>[2x]EDPEV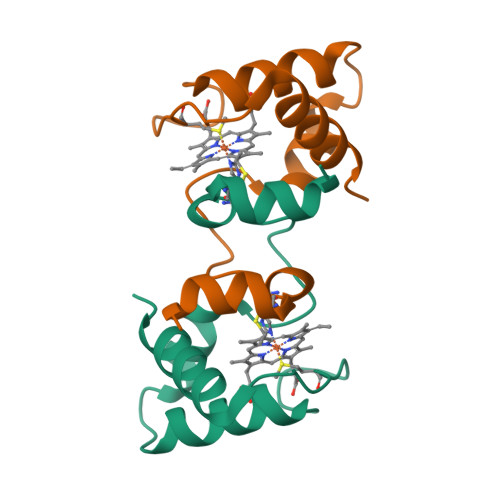LFKNKGCVACHAIDTKMVGPAYKDVAAKFAGQAGAEAELAQRIKNGSQGVWGPIPMPPNAVSDDEAQTLAKWVLSQK>APITAPDITSICKDASSGIGNQEGAIRTRKCCPPSLGKKIKDFQFPNDKKVRMRWPAHKGTKKQVDDYRRAIAAMRALPDDDPRSFVSQAKIHCAYCNGGYTQVDSGFPDIDIQIHNSWLFFPFHRWYLYFYERILGSLIDEPNFALPYWKWDEPKGMPISNIFLGDASNPLYDQYRDANHIEDRIVDLDYDGKDKDIPDQQQVACNLSTVYRDLVRNGVDPTSFFGGKYVAGDSPVANGDPSVGSVEAGSHTAVHRWVGDPTQPNNEDMGNFYSAGYDPVFYIHHANVDRMWKLWKELRLPGHVDITDPDWLNASYVFYDENKDLVRVYNKDCVNLDKLKYNFIENSKE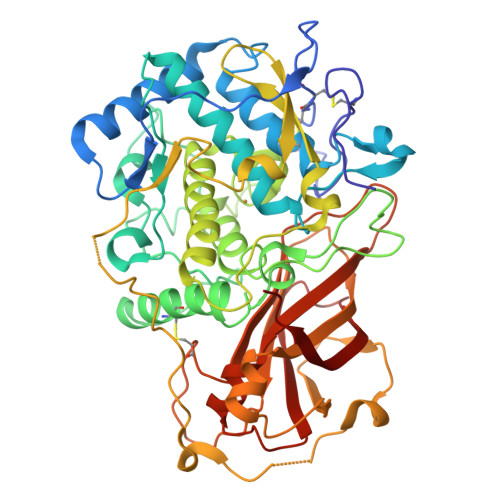VFPWRNSRPPQRRKSAQVATTGDVKTVEQTKFPVRLNQIFKVRVKRPAVNRTEEEKDQANEVLLIKKIKYDSGKFVKFDVFVNDKLKDGVFTTPCDPEYAGGFAQIPHNDKRSMVMTSTARFGLNELLEDTNTEGEEYATVTLVPRTGCEDLTVGEIKIELVPIPKA[4x]>[2x]GSLPVASVSLDTVT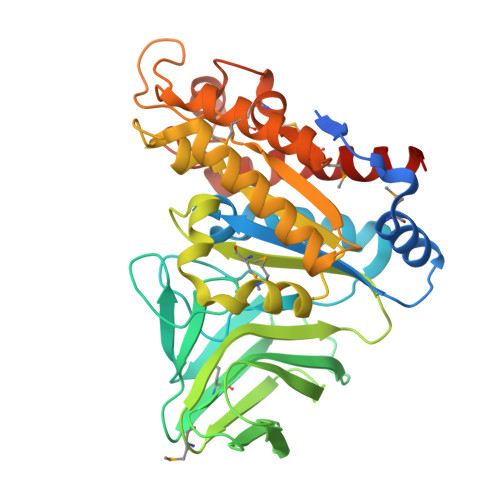VSPSAPYTDTNGLLTDYGNASASPWMKKLQSVAQGSGETFRILQIGDSHTAGDFFTDSLRKRLQKTWGDGGIGWVYPANVKGQRMAAVRHNGNWQSLTSRNNTGDFPLGGILAHTGSGGSMTLTASDGIASKQRVSLFAKPLLAEQTLTVNGNTVSANGGGWQVLDTGAALPLTIHTEMPWDIGFINIENPAGGITVSAMGINGAQLTQWSKWRADRMNDLAQTGADLVILSYGTNEAFNNNIDIADTEQKWLDTVRQIRDSLPAAGILIIGAPESLKNTLGVCGTRPVRLTEVQQMQRRVARQGQTMFWSWQNAMGGICSMKNWLNQGWAAKDGVHFSAKGYRRAAEMLADSLEELVRSAAIRQ> GPLGSMDHDTEVIVKDFNSILEELTFNSRPIITTLTKLAEENISCAQYFVDAIESRIEKCMPKQKLYAFYALDSICKNVGSPYTIYFSRNLFNLYKRTYLLVD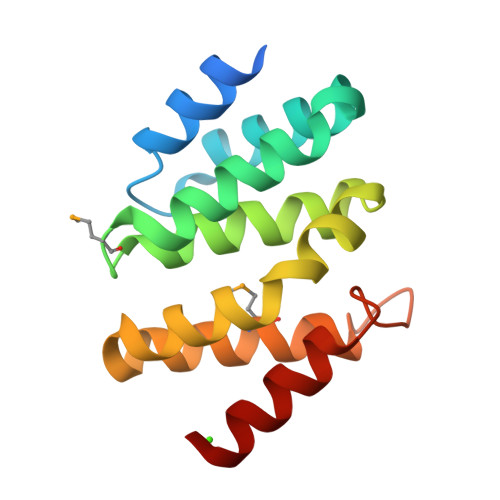NTTRTKLINMFKLWLNPNDTGLPLFEGSALEKIEQFLIKA> SNSGEPAPVLSSPTPTDLSTFLSFPSPEKLLRLGPKVSVLIVQQTDTSDPEKVVSAFLKVASVFRDDASV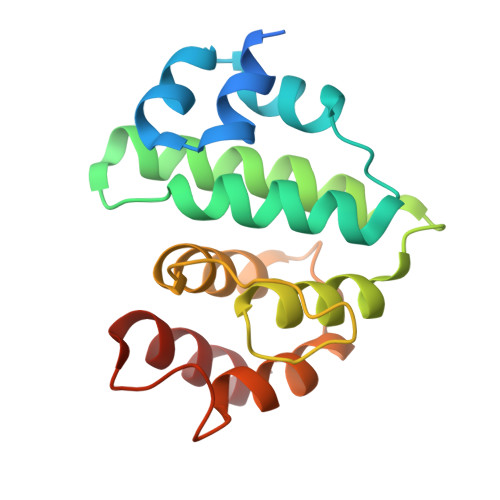KTAVLDAIDALMKKAFSCSSFNSNTFLTRLLIHMGLLKSEDKIKAIPSLHGPLMVLNHVVRQDYFPKALAPLLLAFVTKPNGALETCSFARHNLLQTLYNI>GPMQLEDLKQQLQQAEEALVAKQEVIDKLKEEAAQHAIVMETVPVLKAQADIYKADFQAERQAREKLAEKK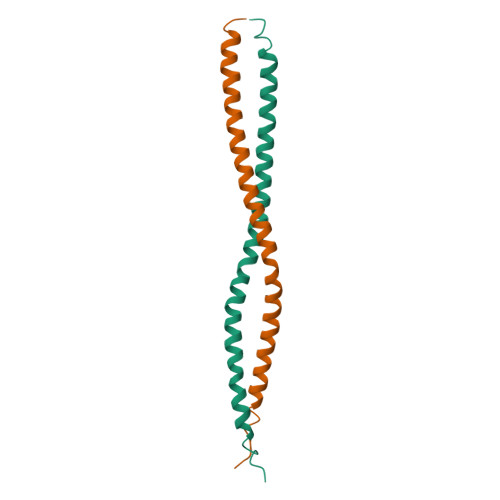ELLQEQLEQLQREYSKLK[2x]> GPAMAEVPSGTVLAEKQELVRHIKDEPASLDPAKAVGLPEIQVIRDLFEGLVNQNEKGEIVPGVATQWKSNDNRIWTFTLRDNAKWADGTPVTAQDFVYSWQRLVDPKTLSPFAWFAALAGINNAQAIIDGKATPDQLGVT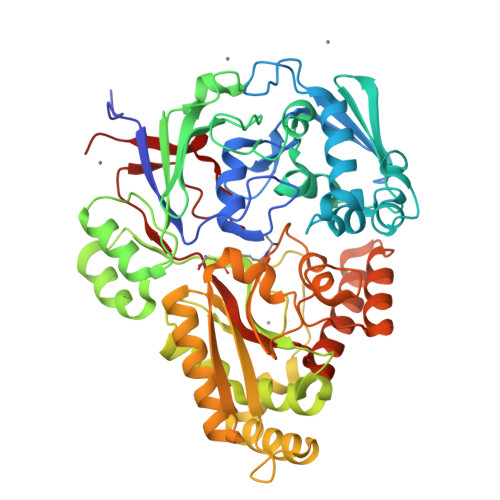AVDAHTLKIQLDKPLPWFVNLTANFAFFPVQKANVESGKEWTKPGNLIGNGAYVLKERVVNEKLVVVPNTHYWDNAKTVLQKVTFLPINQESAATKRYLAGDIDITESFPKNMYQKLLKDIPGQVYTPPQLGTYYYAFNTQKGPTADQRVRLALSMTIDRRLMTEKVLGTGEKPAWHFTPDVTAGFTPEPSPFEQMSQEELNAQAKTLLSAAGYGPQKPLKLTLLYNTSENHQKIAIAVASMWKKNLGVDVKLQNQEWKTYIDSRNTGNFDVIRASWVGDYNEPSTFLTLLTSTHSGNISRFNNPAYDKVLAQASTENTVKARNADYNAAEKILMEQAPIAPIYQYTNGRLIKPWLKGYPINNPEDVAYSRTMYIVKH> DLFTLSFSPDLSIASEAEQLTLQSKDDRLILEHPQPGLRTALEQLKQGNLTLAQLTELVSEQDGVEAGITFASELEKLVDLGWICHSVLPLITAIPIAKDYELNVPDSSWQTTAIALSRFAFLHQDLQQLVLESPRSKSKLVILDWRVGAVIAKLAQSDRGFIFATSADSLLADLSLELEELKRLFALLIATQMMDLEPEDETITQWKFHNLLFHHYTRLGRLDNSRKLNLPVFEHRDRYPYVKPVISTQAIPLVKPDLTALATTDMTLTEAIETRRSIREYSDQPITLAQLGEFLYRCARVKAVYTLPEDPMQVGESTTRPYPSGGALYELEIYPLVHQCGDLAAGLYHYQPLSHTLHPVADWTPEVESLVYDAWRATGQQSIPQIVLIITARFGRLFWKYHDIAYSLILKHVGVLYQTFYLVATAMQLAPSAIGAGNTTKFCQIAGLNPDEEASVGEFSLGAAKP;> MLDLFTLSFSPDLSIASEAEQLTLQSKDDRLILEHPQPGLRTALEQLKQGNLTLAQLTELVSEQDGVEAGITFASELEKLVDLGWICHSVLPLITAIPIAKDYELNVPDSSWQTTAIALSRFAFLHQDLQQLVLESPRSKSKLVILDWRVGAVIAKLAQSDRGFIFATSADSLLADLSLELEELKRLFALLIATQMMDLEPEDETITQWKFHNLLFHHYTRLGRLDNSRKLNLPVFEHRDRYPYVKPVISTQAIPLVKPDLTALATTDMTLTEAIETRRSIREYSDQPITLAQLGEFLYRCARVKAVYTLPEDPMQVGESTTRPYPSGGALYELEIYPLVHQCGDLAAGLYHYQPLSHTLHPVADWTPEVESLVYDAWRATGQQSIPQIVLIITARFGRLFWKYHDIAYSLILKHVGVLYQTFYLVATAMQLAPSAIGAGNTTKFCQIAGLNPDEEASVGEFSLGAAKPQQQS

Cyanobactins are a family of ribosomally synthesized and post-translationally modified peptides (RiPPs; Arnison et al., 2013) from cyanobacteria. The only enzyme function remaining to be solved in the patellamide cluster is that of the FMN-dependent cyanobactin azoline oxidase. The oxidase converts thiazolines to thiazoles, with some enzymes also capable of the oxidation of oxazolines to oxazoles. We have reported the first structure of an oxidase protein from a cyanobactin pathway.

Here, we present ThcOx, the first novel structure to be solved by in-vacuum long-wavelength macromolecular crystallo­graphy on beamline I23 at Diamond Light Source, and its subsequent high-resolution structure solved by molecular replacement. The protein crystals belonged to space group P412121, with two molecules found in the asymmetric unit. Hence, molecular replacement was needed to phase the high-resolution data. The structure is composed of a novel domain and an FMN nitroreductase domain. Each molecule in the asymmetric unit consists of 16 α-helices and 17 β-sheets (structural figures were created using PyMOL v.1.5.0.4 from Schrödinger). The final structure contains residues 3–222 and 233–469 in chain A and 1–222 and 231–473 in chain B. In both monomers, the missing residues are located between α-helices 7 and 8 (the linker between the two domains) and at the N- and C-termini. PISA analysis infers that the dimer is biologically relevant, with each molecule containing a single FMN. The N-terminal domain contains a portion (residues 7–86) which, by visual analysis, supported by Phyre2, possesses the same fold as the leader binding domain of TruD, the so-called ‘peptide-clamp domain’. The remaining residues in domain 1 (87–194) form a second peptide-clamp domain, but its binding site is buried by an interaction with the other clamp domain and thus it is unlikely to be active. The peptide was included as there was evidence that it may bind to the oxidase; however, there was no evidence of any density for the peptide.> DV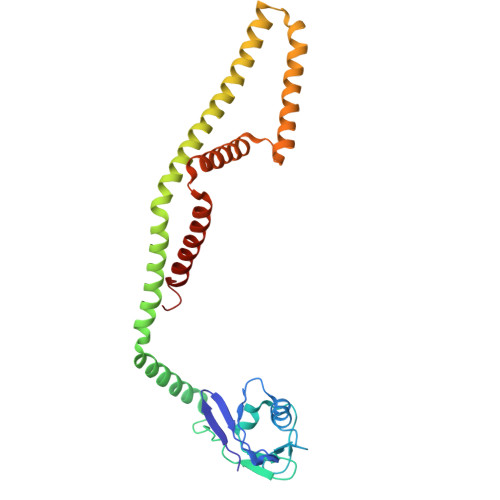TVVYQNGLPVISVRLPSRRERCQFTLKPISDSVGVFLRQLQEEDRGIDRVAIYSPDGVRVAASTGIDLLLLDDFKLVINDLTYHVRPPKRDLLSHENAATLNDVKTLVQQLYTTLCIEQHQLNKERELIERLEDLKEQLAPLEKVRIEISRKAEKRTTLVLWGGLAYMATQFGILARLTWWEYSWDIMEPVTYFITYGSAMAMYAYFVMTRQEYVYPEARDRQYLLFFHKGAKKSRFDLEKYNQLKDAIAQAEMDLKRLRDPLQVH>KFSVLKGKRLFAILRLADGSQPPFGASVTSEKGRELGMVADEGLAWLSGVTPGETLSVNWDGKIQCQVNVPETAISDQ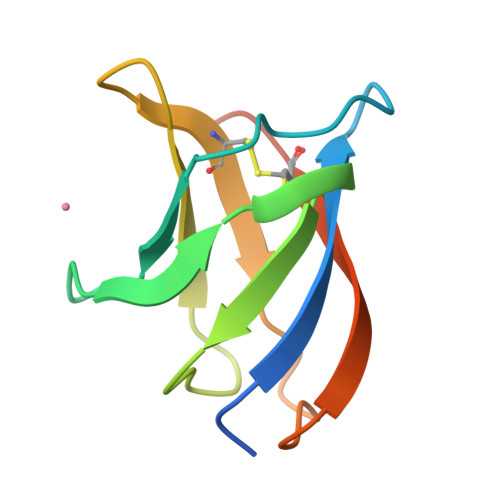QLLLPCTPQKHHHHHH[5x]>SMDLLVPKLTASVTDGAVGVTVDAPVSVTAADGVLAAVTMVNDNGRPVAGRLSPDGLRWSTTEQLGYNRRYTLNATALGLGGAATRQLTFQTSSPAHLTMPYVMPGDGEVVGVGEPVAIRFDENIADRGAAEKAIKITTNPPVEGAFYWLNNREVRWRPEHFWKPGTAVDVAVNTYGVDLGEGMFGEDNVQTHFTIGDEVIATADDNTKILTVRVNGEVVKSMPTSMGKDSTPTANGIYIVGSRYKHIIMDSSTYGVPVNSPNGYRTDVDWATQISYSGVFVHS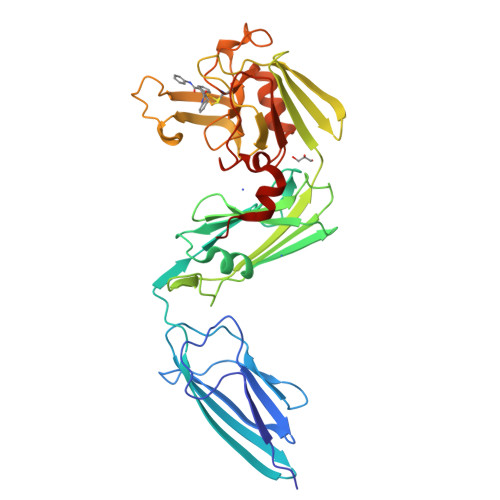APWSVGAQGHTNTSHGCLNVSPSNAQWFYDHVKRGDIVEVVNTVGGTLPGIDGLGDWNIPWDQWRAGNAKA[2x]>CUUGCUGAAGUGCACACAG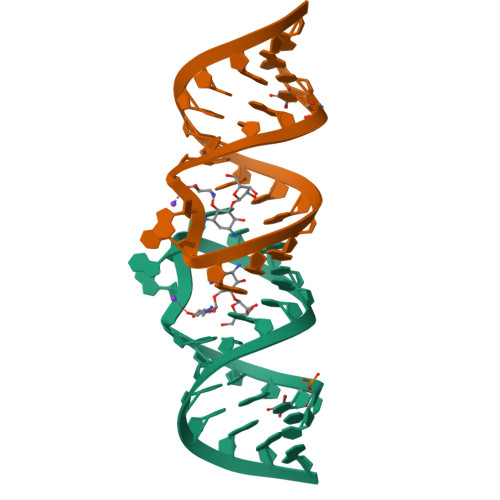CAAG[4x]> SDKKSLMPLVGIPGEIKNRLNILDFVKNDKFFTLYVRALQVLQARDQSDYSSFFQLGGIHGLPYTEWAKAQPQLHLYKANYCTHGTVLFPTWHRAYESTWEQTLWEAAGTVAQRF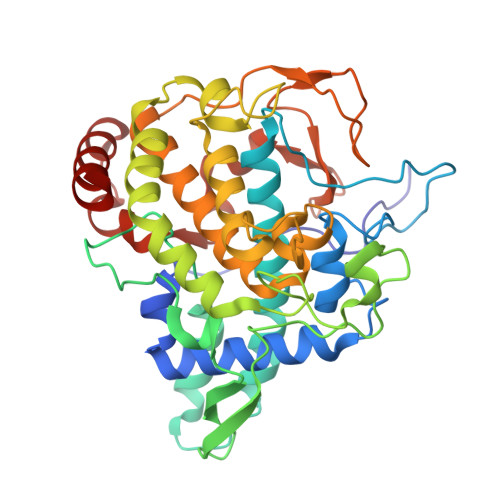TTSDQAEWIQAAKDLRQPFWDWGYWPNDPDFIGLPDQVIRDKQVEITDYNGTKIEVENPILHYKFHPIEPTFEGDFAQWQTTMRYPDVQKQENIEGMIAGIKAAAPGFREWTFNMLTKNYTWELFSNHGAVVGAHANSLEMVHNTVHFLIGRDPTLDPLVPGHMGSVPHAAFDPIFWMHHCNVDRLLALWQTMNYDVYVSEGMNREATMGLIPGQVLTEDSPLEPFYTKNQDPWQSDDLEDWETLGFSYPDFDPVKGKSKEEKSVYINDWVHKHYG> GGSHTADRWRVSLDVNHFAPDELTVKTKDGVVEITGKHAARQDEHGYISR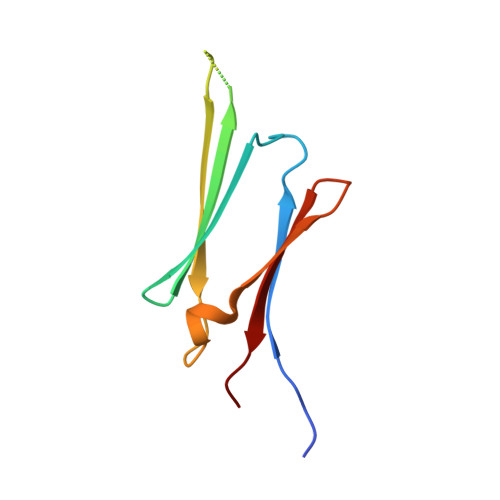CFTRKYTLPPGVDPTQVSSSLSPEGTLTVEAPMPK> EPFWADLQPRVAFVERGGSLWLNCSTNCPRPERGGLETSLRRNGTQRGLRWLARQLVDIREPETQPVCFFRCARRTLQARGLIRTFQRPDRVELMPLPPWQPVGENFTLSCRVPGAGPRASLTLTLLRGAQELIRRSFAGEPPRARGAVLTATVLARREDH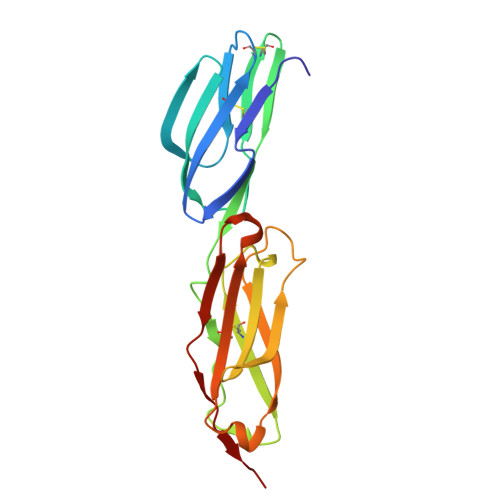GANFSCRAELDLRPHGLGLFENSSAPRELRTFSLS> MTTITTYPGVYIEEDASLSLSVSSSATAVPVFAVAGDNPLISGKPYIRISNWLEYLTLKNEQFDPANTLDISLRAYFINGGGYCYLVQTTDLEKQVPKLDDVTLLVAAGENITTAVSTLCKPGKGLFAIFDGPTTELKSDGTSNSDYDPNPFAAVYYPWLTADWTTTIDIPPSAAIAGVYCSVDSTRGVWKAPANVPIQGGLQPKYPVTDDLQAQYNQGKALNMIRTFPKSGTLVWGARTLEDNDNWRYIPVRRLFNSAERDIKNAMSFAVFEPNSQPTWERVRSAVNNYLYSLWQQGGLAGNKPDDAYFVQIGKDITMTDDDI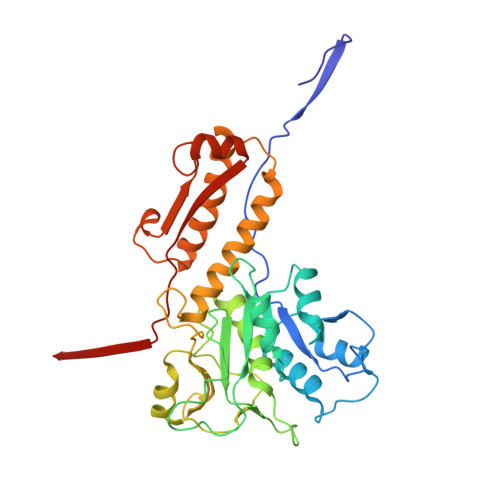KQGKMIIKIGMAAVRPAEFIILQFTQNTAQ>[2x]MVSGVGGSGGGRGGGRGGEEEPSSSHTPNNRRGGEQAQSSGTKSLRPRSNTESMSKAIQQYTVDARLHAVFEQSGESGKSFDYSQSLKTTTYGSSVPEQQITAYLSRIQRGGYIQPFGCMIAVDESSFRIIGYSENAREMLGIMPQSVPTLEKPEILAMGTDVRSLFTSSSSILLERAFVAREITLLNPVWIHSKNTGKPFYAILHRIDVGVVID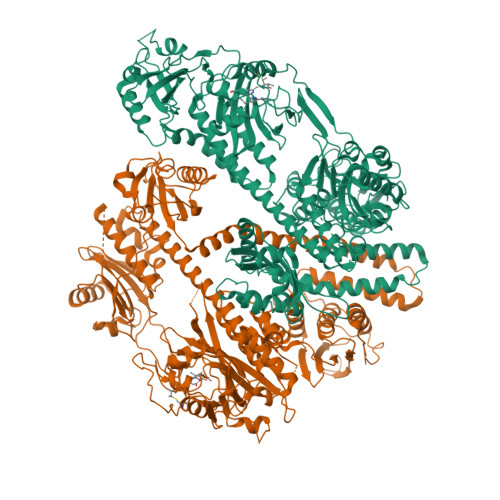LEPARTEDPALSIAGAVQSQKLAVRAISQLQALPGGDIKLLCDTVVESVRDLTGYDRVMVYKFHEDEHGEVVAESKRDDLEPYIGLHYPATDIPQASRFLFKQNRVRMIVDCNATPVLVVQDDRLTQSMCLVGSTLRAPHGCHSQYMANMGSIASLAMAVIINGNEDDGSNVASGRSSMRLWGLVVCHHTSSRCIPFPLRYACEFLMQAFGLQLNMELQLALQMSEKRVLRTQTLLCDMLLRDSPAGIVTQSPSIMDLVKCDGAAFLYHGKYYPLGVAPSEVQIKDVVEWLLANHADSTGLSTDSLGDAGYPGAAALGDAVCGMAVAYITKRDFLFWFRSHTAKEIKWGGAKHHPEDKDDGQRMHPRSSFQAFLEVVKSRSQPWETAEMDAIHSLQLILRDSFKESEAAMNSKVVDGVVQPCRDMAGEQGIDELGAVAREMVRLIETATVPIFAVDAGGCINGWNAKIAELTGLSVEEAMGKSLVSDLIYKENEATVNKLLSRALRGDEEKNVEVKLKTFSPELQGKAVFVVVNACSSKDYLNNIVGVCFVGQDVTSQKIVMDKFINIQGDYKAIVHSPNPLIPPIFAADENTCCLEWNMAMEKLTGWSRSEVIGKMIVGEVFGSCCMLKGPDALTKFMIVLHNAIGGQDTDKFPFPFFDRNGKFVQALLTANKRVSLEGKVIGAFCFLQIPSPELQQALAVQRRQDTECFTKAKELAYICQVIKNPLSGMRFANSLLEATDLNEDQKQLLETSVSCEKQISRIVGDMDLESIEDGSFVLKREEFFLGSVINAIVSQAMFLLRDRGLQLIRDIPEEIKSIEVFGDQIRIQQLLAEFLLSIIRYAPSQEWVEIHLSQLSKQMADGFAAIRTEFRMACPGEGLPPELVRDMFHSSRWTSPEGLGLSVCRKILKLMNGEVQYIRESERSYFLIILELPVPRKRPLSTASGSGDMMLMMPY>[2x]ASRAPGQGGGAAVEKDPIKLWDRYVEW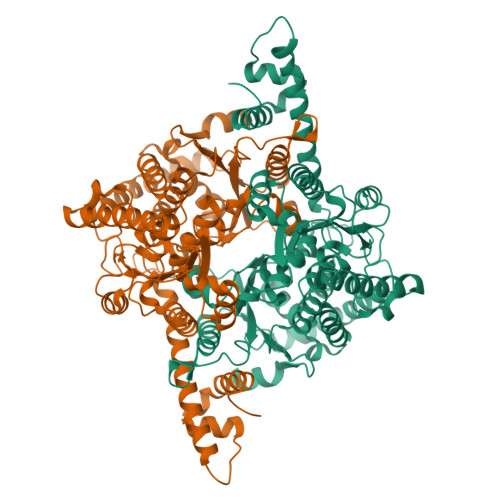LYQHKQLGLFVDVSRMGFTDDFLLQMEPLMQRAFVAMGELEKGAIANPDEGRMVGHYWLRDPGLAPNSFLRTKIEKTVDHILAFSQDIVSGKIKPPSSQAGRFTQILSIGIGGSSLGPQFVSEALAPDNPPLKIRFIDNTDPAGIDHQIAQLGEELKSTLVIVISKSGGTPETRNGLLEVQKAFRDAGLDFSKQGVAITQENSLLDNTARIEGWLDRFPMFDWVGGRTSELSAVGLLPAALQGIDVKEMLVGAALMDEETRNTVVKENPAALLALSWYWATDGIGSKDMVVLPYKDSLLLLSRYLQQLVMESLGKEFDLDGNRVNQGLTVYGNKGSTDQHAYIQQLREGVHNFFVTFIEVLRDRPPGHDWELEPGVTCGDYLFGMLQGTRSALYSNDRESISVTVEEVTPRAVGALVALYERAVGIYASLVNINAYHQPGVEAGKKAAGEVLALQKRVLTVLNEASCKDPAEPLTLEQIADRCHCPEDIEMIYKIIQHMAANDRALIAEGSCGSPRSVKVYLGECNVDDV>[4x]SKKIGLFYGTQTGKTESVAEIIRDEFGNDVVTLHDVSQAEVTDLNDYQYLIIGCPTANIGELQSDWEGLYSELDDVDFNGKLVAYFGTGDQIGYADNFQDAIGILEEKISQR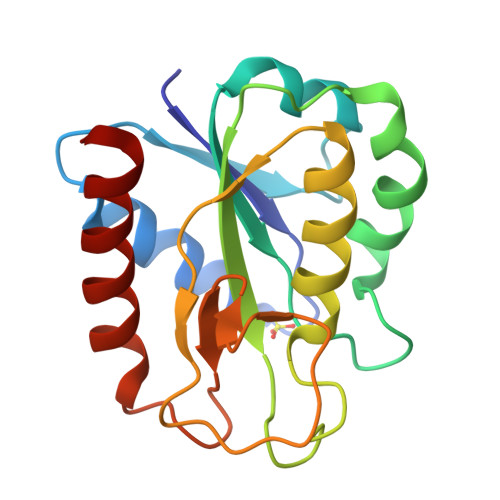GGKTVGYWSTDGYDFNDSKALRNGKFVGLALDEDNQSDLTDDRIKSWVAQLKSEFGL>DAAKLLHRERMERVTAFLSYKKISPELQRRILEYFDYLWETRRGYEEREVLKE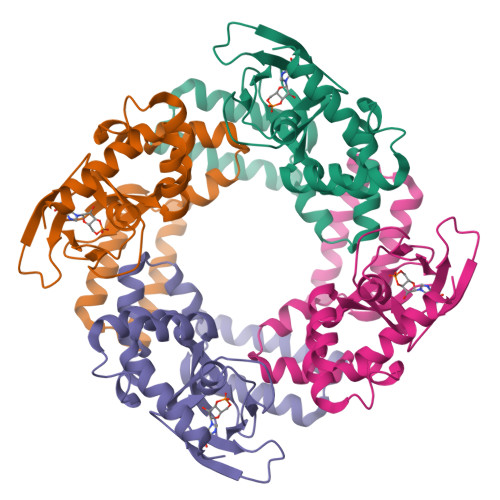LPHPLRLAVAMEIHGDVIEKVPLFKGAGEDFIRDIILHLEPVIYGPGEYIIRAGELGSDVYFINRGSVEVLSADEKTRYAILSEGQFFGEMALILRAPRTATVRARTFCDLYRLDKETFDRILSRYPEIAAQIQELAVRRKEELE[2x]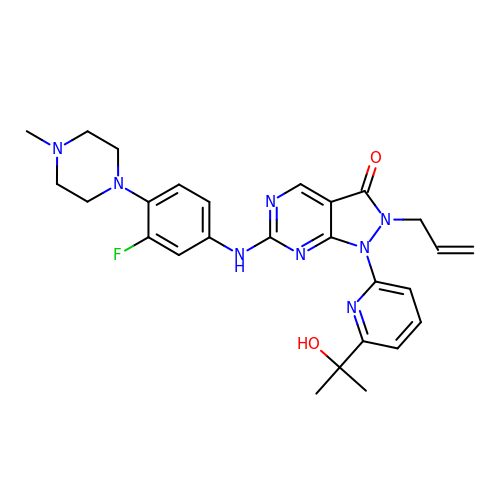6-{[3-fluoro-4-(4-methylpiperazin-1-yl)phenyl]amino}-1-[6-(2-hydroxypropan-2-yl)pyridin-2-yl]-2-(prop-2-en-1-yl)-1,2-dihydro-3H-pyrazolo[3,4-d]pyrimidin-3-one | C27 H31 F N8 O2 | LAMATIDTONUKGC-UHFFFAOYSA-N> MRGSHHHHHHGSGLSSLQSDPAGCVRPPAPNLAGAVEFNDVKTLLREWITTISDPMEEDILQVV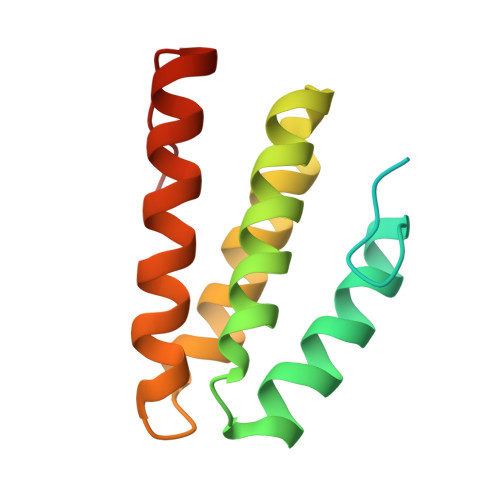KYCTDLIEEKDLEKLDLVIKYMKRLMQQSVESVWNMAFDFILDNVQVVLQQTYGSTLKVT3'-3"-DICHLOROPHENOL-1,8-3H-BENZO[DE]ISOCHROMEN-1-ONE | C24 H14 Cl2 O4 | 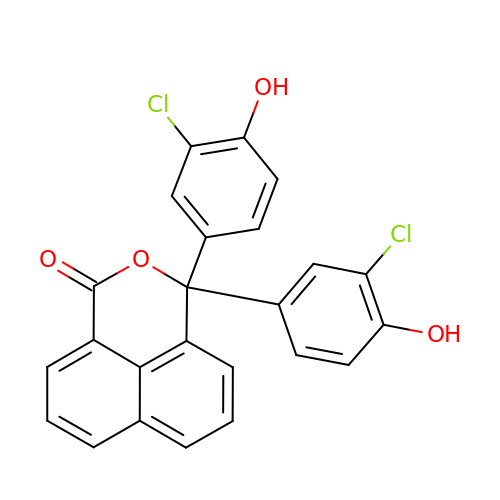HCQHFJBXXMFZHF-UHFFFAOYSA-N> STQACPQPKTLDEFTIIQNLQPQYQ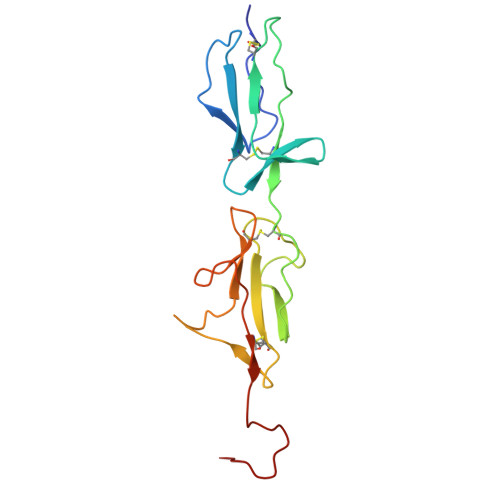FRDYFIATCKQGYQLIEGNQVLHSFTAVCQDDGTWHRAMPRCKIKDCGQPRNLPNGDFRYTTTMGVNTYKARIQYYCHEPYYKMQTRAGSRESEQGVYTCTAQGIWKNEQKGEKIPRCLPVCGKPVNPVEQRQR> DFPAGTTPNEHNINGADYPRIGEDRRVHFRIHAPNAQKVEISFRGEMTKEADGYWSLVSKEPEVIGFHYYQVIIDGVSAADPNGKPFFGMGKWVSGIEIPEKGVDYYSIKNVPHGLISQSWYYSDIRKEWRRCIVYTPAEYDKNPTKKYPVLYLQHGMGENETSWANQGKMNFIMDNLIAEGKAKPMIVVMDNGNIEVFKTNSGETPEDARKRFGAEFPAILVNEIIPHIESNFRTLTDRDNRAMAGLSWGGLLTFNTTLNNLDKFAYIGGFSGAGSIDLKQLDTVYGGVFK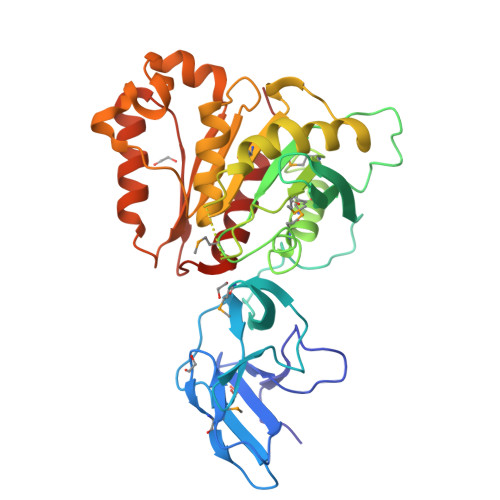NRKAFNDKVHVFFLGIGSEEHPERTKNLSDGLQAAGINTIYYESPGTAHEFLTWRRCLKEFAPLLFKT>MSLVNRKQLEKMANVRFRVQEDEYVAILDALEEYHNMSENTVVEKYLKLKDINSLTDTYIDTYKKSGRNKALKKFKEYLVIEILELKNSNLTPVEKNLHFIWIGGQINDTAINYINQWKDVNSDYNVNVFYDSNAFLINTLKKTIIESASNDTLESFRENLNDPEFNHTAFFRKRMQIIYDKQQNFINYYKAQKEENPDLIIDDIVKTYLSNEYSKDIDELNAYIEESLNKVTENSGNDVRNFEEFKTGEVFNLYEQELVERWNLAGASDILRVAILKNIGGVYLDVDMLPGIHPDLFKDINKPDSVKTAVDWEEMQLEAIMKHKEYIPEYTSKHFDTLDEEVQSSFESVLASKSDKSEIFLPLGDIEVSPLEVKIAFAKGSIINQALISAKDSYCSDLLIKQIQNRYKILNDTLGPIISQGNDFNTTMNNFGESLGAIANEENISFIAKIGSYLRVGFYPEANTTITLSGPTIYAGAYKDLLTFKEMSIDTSILSSELRNFEFPKVNISQATEQEKNSLWQFNEERAKIQFEEYKKNYFE[2x];>[2x]DPPPSETHKLVVVGGGGVGKSALTIQFIQSYFVSDYDPNIEDSYTKICSVDGIPARLDILDTAGQEEFGAMREQYMRAGHGFLLVFAINDRQSFNEVGKLFTQILRVKDRDDFPVVLVGNKADLESQRQVPRSEASAFGASHHVAYFEASAKLRLNVDEAFEQLVRAVRKYQEQEL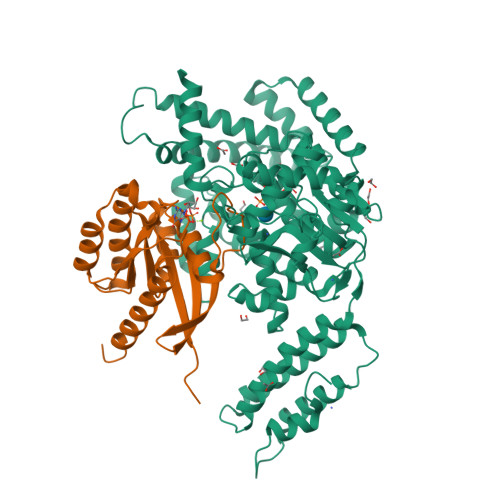PPS> GSSMGSLNQDATILRQAKLGLSDPAQSLSSWSDNNDVTPCKWLGVSCDATSNVVSVDLSSFMLVGPFPSILCHLPSLHSLSLYNNSINGSLSADDFDTCHNLISLDLSENLLVGSIPKSLPFNLPNLKFLEISGNNLSDTIPSSFGEFRKLESLNLAGNFLSGTIPASLGNVTTLKELKLAYNLFSPSQIPSQLGNLTELQVLWLAGCNLVGPIPPSLSRLTSLVNLDLTFNQLT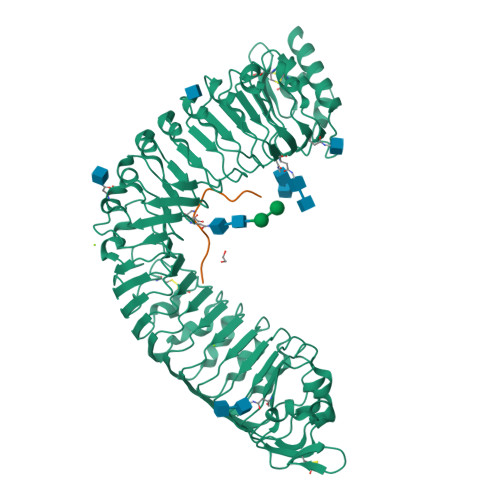GSIPSWITQLKTVEQIELFNNSFSGELPESMGNMTTLKRFDASMNKLTGKIPDNLNLLNLESLNLFENMLEGPLPESITRSKTLSELKLFNNRLTGVLPSQLGANSPLQYVDLSYNRFSGEIPANVCGEGKLEYLILIDNSFSGEISNNLGKCKSLTRVRLSNNKLSGQIPHGFWGLPRLSLLELSDNSFTGSIPKTIIGAKNLSNLRISKNRFSGSIPNEIGSLNGIIEISGAENDFSGEIPESLVKLKQLSRLDLSKNQLSGEIPRELRGWKNLNELNLANNHLSGEIPKEVGILPVLNYLDLSSNQFSGEIPLELQNLKLNVLNLSYNHLSGKIPPLYANKIYAHDFIGNPGLCVDLDGLCRKITRSKLEGSENLYFQ;> YPKGVPIPPSAPSKRHN>MLEARFQQAALLKKLLDAIKELVTDANFDCNDNGISLQAMDSSHVALVSMLIKSDGFEPYRCDRNIALGINLNALSKVLRCAQNEDLVTLKAEDTPEVLNLVFESEKNDRISDYDVKLMDID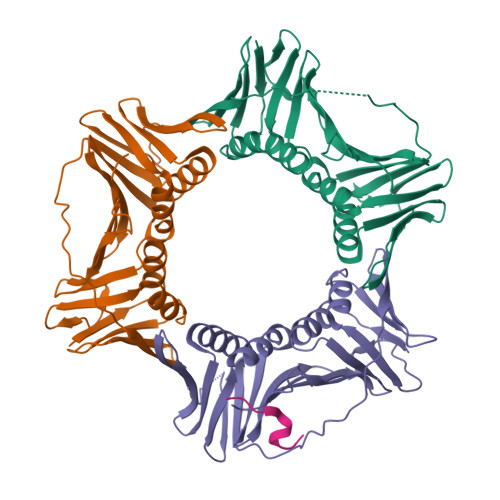QEHLGIPDIEYDATITMPAAEFQRITRDLLTLSDSVTINASKEGVRFSCKGDIGNGSTTLKQHTDLSDQDQSIEISLTQAVTLTFSLKYLAQFTKATPLATRVTLSMSNDVPLLVEYKMESGFLRFYLAPKIGEEDEE[3x];> IQGSLMDVGM>AHGRIELIIGPMFAGKTTELMRRVQRHKHAQRSCYIIKYTGDTRYSEGAITSHDQRALTANVSVSNLHDVGDEWRKYDVIAVDEGQFFPDVAAFCSKAADSGKVVIVSALDADYLQEPFEEICLLVSRADSVVKLSAVCMECHNRKASFTYRTVKSDERKLVGGSDMYMSVCRSCYETKRNM[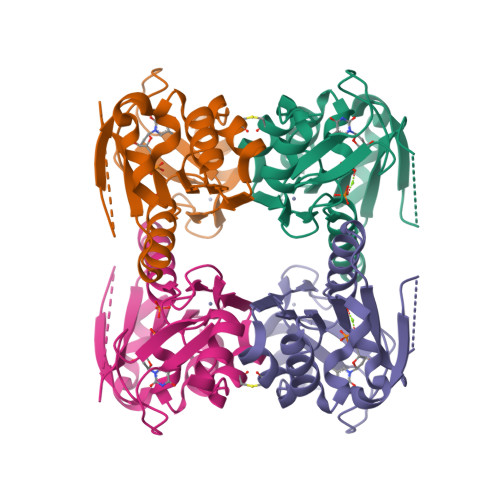2x]>MGHHHHHHGRAMNNPAIKRIGNHITKSPEDKREYRGLELANGIKVLLISDPTTDKSSAALDVHIGSLSDPPNIAGLSHFLQHMLFLGTKKYPKENEYSQFLSEHAGSSNAFTSGEHTNYYFDVSHEHLEGALDRFAQFFLSPLFDESAKDREVNAVDSEHEKNVMNDAWRLFQLEKATGNPKHPFSKFGTGNKYTLETRPNQEGIDVRQELLKFHSAYYSSNLMAVVVLGRESLDDLTNLVVKLFSEVENKNVPLPEFPEHPFQEEHLKQLYKIVPIKDIRNLYVTFPIPDLQKYYKSNPGHYLGHLIGHEGPGSLLSELKSKGWVNTLVGGQKEGARGFMFFIINVDLTEEGLLHVEDIILHMFQYIQKLRAEGPQEWVFQELKDLNAVAFRFKDKERPRGYTSKIAGILHYYPLEEVLTAEYLLEEFRPDLIEMVLDKLRPENVRVAIVSKSFEGKTDRTEEWYGTQYKQEAIPDEVIKKWQNADLNGKFKLPTKNEFIPTNFEILPLEKEATPYPALIKDTAMSKLWFKQDDKFFLPKANLNFEFFSPFAYVDPLHSNMAYLYLELLKDSLNEYAYAAELAGLSYDLQNTIYGMYLSVKGYNDKQPILLKKIIEKMATFEIDEKRFEIIKEAYMRSLNNFRAEQPHQH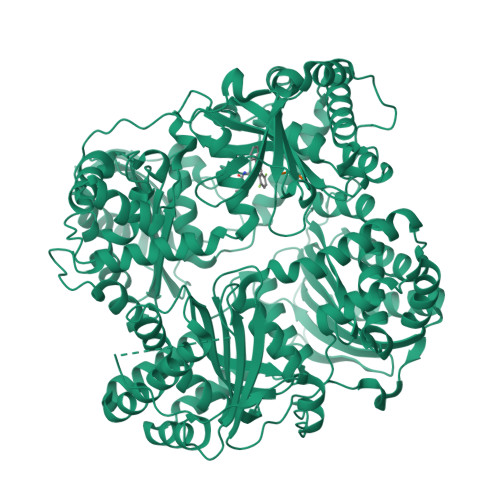AMYYLRLLMTEVAWTKDELKEALDDVTLPRLKAFIPQLLSRLHIEALLHGNITKQAALGIMQMVEDTLIEHAHTKPLLPSQLVRYREVQLPDRGWFVYQQRNEVHNNSGIEIYYQTDMQSTSENMFLELFAQIISEPAFNTLRTKEQLGYIVFSGPRRANGIQGLRFIIQSEKPPHYLESRVEAFLITMEKSIEDMTEEAFQKHIQALAIRRLDKPKKLSAESAKYWGEIISQQYNFDRDNTEVAYLKTLTKEDIIKFYKEMLAVDAPRRHKVSVHVLAREMDSNPVVGEFPAQNDINLSQAPALPQPEVIQNMTEFKRGLPLFPLVKPHINFMAAKL[2x];>[2x]AAA> RELGLGAASAIEQKASAFFSRLTDVQQRQLEKQGLLASRFYRFLVISLMEKEGTFTYYDFYVWRKGCLAYLKAAEEEMQGIVGKSARKLADLGWEKLRPSTSPEFKEMELHLKILSHFTPEELSRDTAEQFTSAAIKNIAKAAETSVKNVKNVLLGHAIALTDRTWYMRLMEMQRPIPQ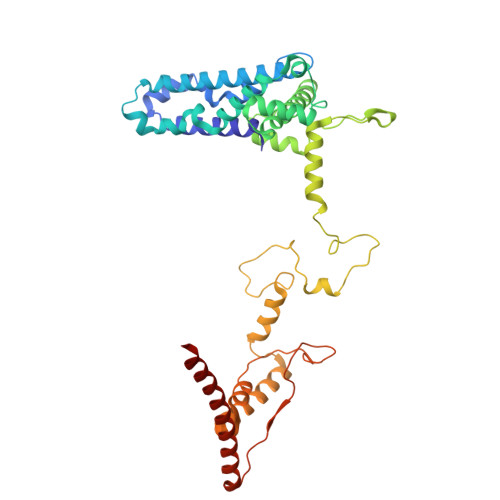SVEDYLLLAETDRPYMIRLPYGEKFYNYELEEALAKKRASERHKSQRDVPRLGRKQHRIRRLFVPNARVAFDRWARIPHARLDAYGNFLYRLNQPAKGAAAVARAAEREKLRVEMSENAEFYSDAALSASRITLNNLPPGAFRRRTGMQRKSGEIHHVAPPRDPVLRELFAAAIQREKDEKRNRERRAQEDAAAAEK> SGMENFILYEEIGRGSKTVVYKGRRKGTINFVAILCTDKC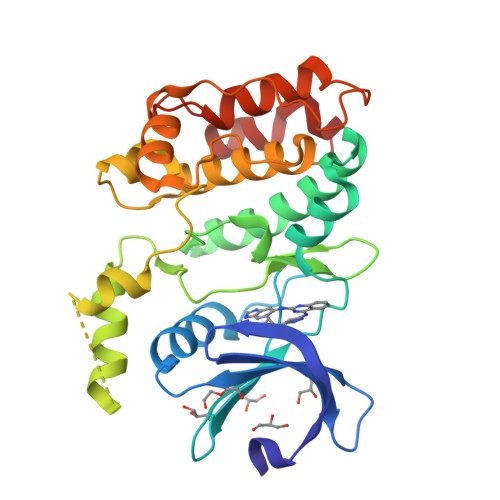KRPEITNWVRLTREIKHKNIVTFHEWYETSNHLWLVVELCTGGSLKTVIAQDENLPEDVVREFGIDLISGLHHLHKLGILFCDISPRKILLEGPGTLKFSNFCLAKVEGENLEEFFALVAAEEGGGDNGENVLAASMKSRVKGSPVYTAPEVVRGADFSISSDLWSLGCLLYEMFSGKPPFFSESISELTEKILCEDPLPPIPKDSSRPKASSDFINLLDGLLQRDPQKRLTWTRLLQHSFWKKAFA> MGSSHHHHHHSSGLVPRGSTDDGEKYSTVERAVKSVDPPATFKPKDEQVFYPNGKPNHQFLKQHFIHEGRLHEHQAIQILKQATHLLSKE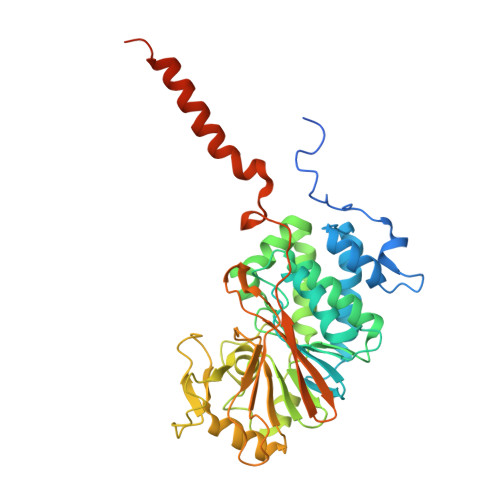PNLLSVPAPVTICGDVHGQYYDLMKLFEVGGDPASTKYLFLGDYVDRGSFSIECLLYLYSLKINYPDTFWMLRGNHECRHLTEYFTFKNECLHKYSEELYEECLVSFNALPLAAIMNEQFFCVHGGLSPQLTSLDSLRKLHRFREPPTKGLMCDLLWADPIEEYDDDNLDQEYVTNVVRGCSFAFTYKAACKFLDRTKLLSVIRAHEAQNAGYRMYKRTKTMGFPSLLTMFSAPNYLDSYNNKAAVLKYENNVMNIRQFNASPHPYWLPHFMDVFTWSLPFVGEKVTDMLVSILNVCTEEELDEDLPFSEAEIGVTPTTTT> RDRAAK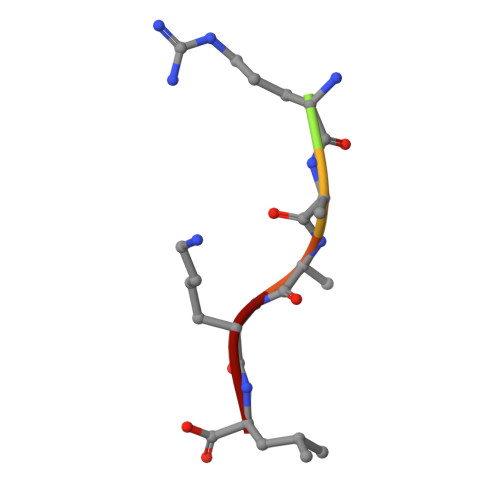L>TPMTNPFPQDFLWGVATAGHQVEGNNVNSDVWFLEHLPGTIFAEPSGDAVDHYHRYREDIALIAGLGFTSYRFSVEWARIEPEEGHFSVAALDHYKRVLEACREHGLTPVVTFHHFASPLWLLRSGGWEGERTPELFARYCGRVMAHLGDLIGVACTLNEPNLPWLLESFGIGGEAPENRGKVPMWAAAAQRLGVDASTVAPFQFCSTEAGFNVKLAAHKAATEAIKAHRPDLRVGWTLANSDIQSVPGGEEIAAQVR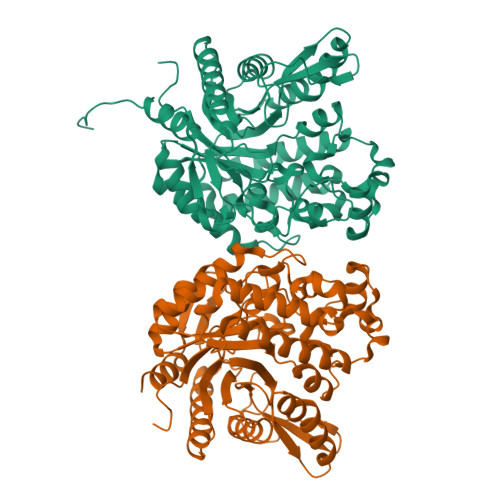RDVNERFLEASRGDDFVGIQTYGRTVYGPDGHAPAPEGVAVNQMGEEIYPQALEATIREAWRVAGIPVMVTENGLATEDDTQRVAYLRTAVDGVASCLADGIDVRGYIAWTAFDNFEWIFGYGPKFGLIAVDRSTQERTPKESARWLGNFARQQAPAEAPQPAKLAAALEHHHHHH[2x]> MRFINQAASDRAVINAGGRRFETLFSTLHRYPDTPFAQLFPLPGRGARQHRGREFFLDVT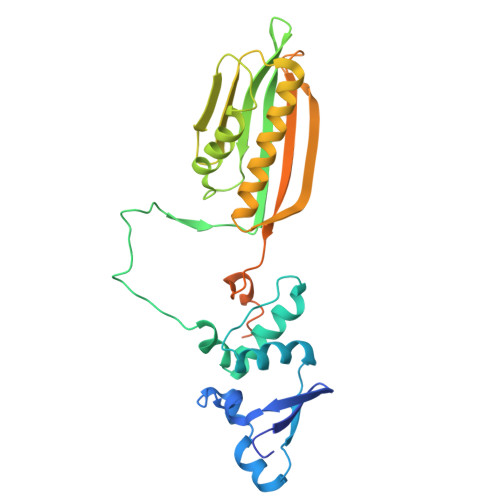PHVFEYILGFLRTNQLNLPAENLQIRAEVVYSMNQWGLLEHAFPPEVIEDGEGCSTGGAVVKLPDVCVVQVCDHMQHDQGVKRHALTITYGADGFQLRSLIRRVRRDLERQLSSTYWQCYQTNERAAFFVTTKVANGTADLLTTSVTQQLVEHTESMGYSLASSYVTLSPDVVHTSVRMLIHNFTFRRSRRVEVEPGDGIALGEGSETIEAEPNIPTMHVGPRREPLNAAESIPPRNERAVNIWTVD>[4x]SNAMVMDDDITVQPIRGVQPRPAGSHEPFAVPSRAGQHGKRPDGEDSADISLSQGAQAAALLFSAAMDQI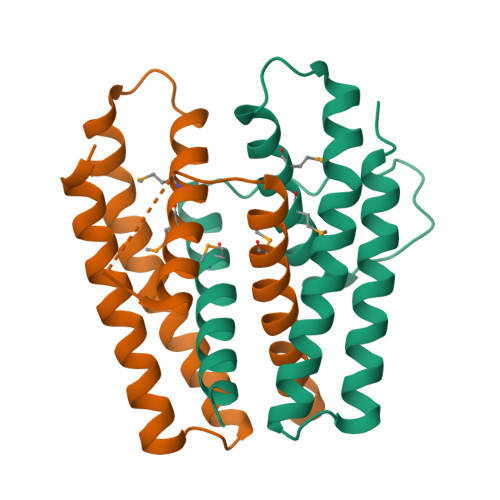SRLAELDIEPVRLPESELTGDSHSQHLLLGMEILMELYRQQHPDWTAPAIRQAFAPLARAGLERGYQEACQVLRQLNVYTPAVAGQLQGLLLLTQRLFEERLQIA>MRGSHHHHHHGSMMSEIIAVANQKGGVGKTTTAVNLAASLAVHEKKILLIDFDPQANATSSLGFRRDKIDYDIYHVLIGRKQISQVILKTQMPFLDLVPSNLGLAGFEKTFYDSQDENKRGELMLKNALESVVGLYDYIIIDSPPALGPLTINSLSAAHSVIIPIQCEFFALEGTKLLLNTIRMLQKSTNPKLKIRGFLPTMHVPQLNLT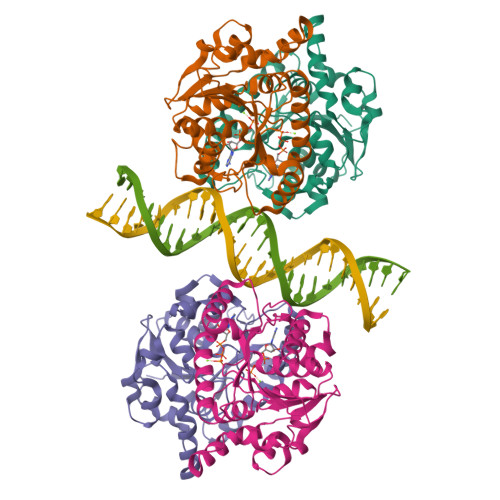KGVLAELFKYFDSEFFRDSATGEYIMIPKSVKLAESPSFGKPILLYDIKSNGSIAYQKLAQSILQG[4x]> ETQNLNAGWTDTAHGSGIIPMKTDLELDFSLPSSASYTYRRQLQNPANEQEKIPFHLQLSKQVIHAEIQHLGHWMDATFNLKTAFHCYGSCEKYAYPWQTAGCFIEKDYEYETGWGCNPPDCPGVGTGCTACGVYLDKLKSVGKVFKIVSLRYTRKVCIQLGTEQTCKTVDSNDCLITTSVKVCLIGTISKFQPSDTLLFLGPLQQGGLIFKQWCTTTCQFGDPGDIMSTPTGMKCPELNGSFRKKCAFATTPVCQFDGNTISGYKRMIATKDSFQSFNVTEPHISTSALEWIDPDSSLRDHINVIVSRDLSFQDLSETPCQIDLATASIDGAWGSGVGFNLVCTVSLTECSAFLTSIKACDAAMCYGSTTANLVRGQNTIHIVGKGGHSGSKFMCCHDTKCSSTGLVAAAPHLDRVTGYNQADSDKIF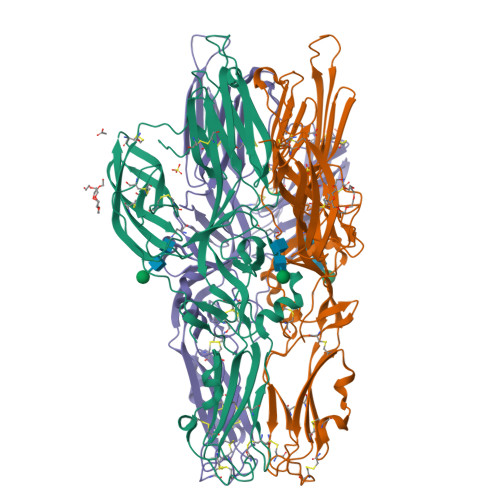DDGAPECGMSCWFKKSGEW>[2x]MALVYDAEFVGSEREFEEERETFLKGVKAYDGVLATRYLMERSSSA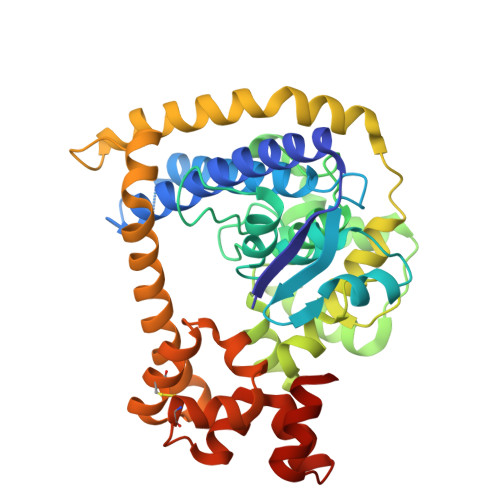KNDEELLELHQNFILLTGSYACSIDPTEDRYQNVIVRGVNFDERVQRLSTGGSPARYAIVYRRGWRAIAKALDIDEEDVPAIEVRAVKRNPLQPALYRILVRYGRVDLMPVTVDEVPPEMAGEFERLIERYDVPIDEKEERILEILRENPWTPHDEIARRLGLSVSEVEGEKDPESSGIYSLWSRVVVNIEYDERTAKRHVKRRDRLLEELYEHLEELSERYLRHPLTRRWIVEHKRDIMRRYLEQRIVECALKLQDRYGIREDVALCLARAFDGSISMIATTPYRTLKDVCPDLTLEEAKSVNRTLATLIDEHGLSPDAADELIEHFESIAGI> MRKELVFVLLALFL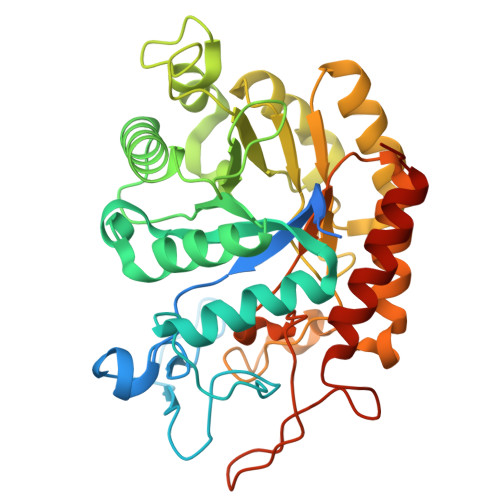CAGCNGNKKKMNGEHDLDAANITLDDHTISFYYNWYGNPSVDGEMKHWMHPIALAPGHSGDVGAISGLNDDIACNFYPELGTYSSNDPEIIRKHIRMHIKANVGVLSVTWWGESDYGNQSVSLLLDEAAKVGAKVCFHIEPFNGRSPQTVRENIQYIVDTYGDHPAFYRTHGKPLFFIYDSYLIKPAEWAKLFAAGGEISVRNTKYDGLFIGLTLKESELPDIETACMDGFYTYFAATGFTNASTPANWKSMQQWAKAHNKLFIPSVGPGYIDTRIRPWNGSTTRDRENGKYYDDMYKAAIESGASYISITSFNEWHEGTQIEPAVSKKCDAFEYLDYKPLADDYYLIRTAYWVDEFRKARSASEDVQ> MKKITLLLA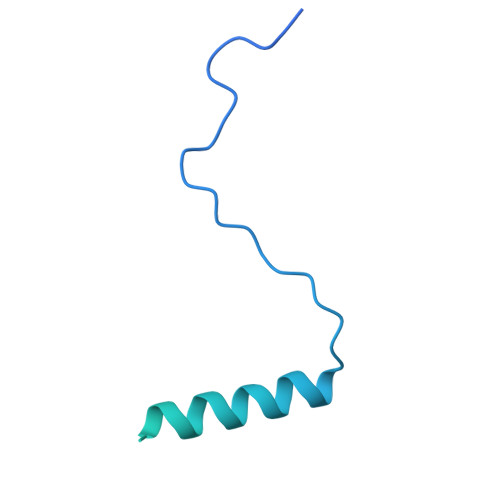GSALLLSGCAGVKSSFDCDATTSDTCMTMTKANQLARDKAAKQAGKPAAGGLPSLVNLPATSAVEVPSASRSAVTPPSGTRTVSTTPPVSAGTSAGVNTNTTTSTLTPRPVAGTPVTTTPSSVAYRPVVSVVTPTPSCQNVRCDNPGTVHPQRSRDQIATVWIAPWVDSDNAFHQPGRVSFVVSPADWVLPARVN>MNKLAVLYAEHIATLQKRTREIIERENLDGVVFHSGQAKRQFLDDMYYPFKVNPQFKAWLPVIDNPHCWIVANGTDKPKLIFYRPVDFWHKVPDEPNEYWADYFDIELLVKPDQVEKLLPYDKARFAYIGEYLEVAQALGFELMNPEPVMNFYHYHRAYKTQYELACMREANKIAVQGHKAARDAFFQGKSEFEIQQAYLLATQHSENDNPYGNIVALNENCAILHYTHFDRVAPATHRSFLIDAGANFNGYAADITRTYDFTGEGEFAELVATMKQHQIALMNQLAPGKLYGELHLDCHQRVAQTLSDFNIVDLSADEIVAKGITSTFFPHGLGHHIGLQVHDVGGFMADEQGAHQEPPEGHPFLRCTRKIEANQVFTIEPGLYFIDS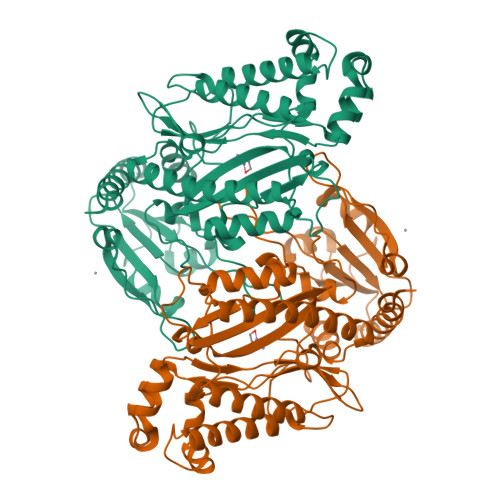LLGDLAATDNNQHINWDKVAELKPFGGIRIEDNIIVHEDSLENMTRELRLRLTTHSLRGLSAPQFSINDPAVMSEYSYPSEPLSYEEEIKKSTFIVHVRTRRILVRRRTLSPILIAVTPMPAITAGLM[3x]>[6x]MNDSATENRTVVVERQISHPPEKLWRALTQPHLIEEWLMKNDFKPAVGHRFNISADWGGVLDCEVLAVEPNKTLSYTWNLAHQDPAFDLRSVVTF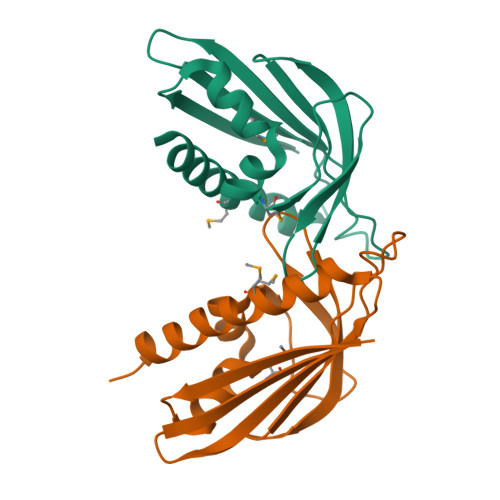TLTPTPTGTHLRMEQSGFRPDQRRAYGGAKMGWPQFFEKLEQLLDRTDLEHHHHHH>S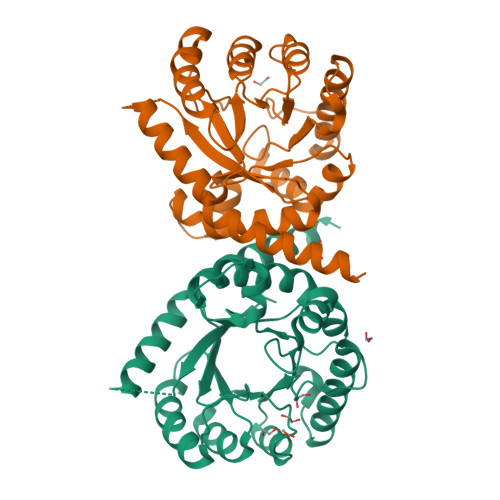NAMTKTKIMGILNVTPDSFSDGGKFNNVETAINRVKAMIDEGADIIDVGGVSTRPGHEMVTLEEELNRVLPVVEAIVGFDVKISVDTFRSEVAEACLKLGVDMINDQWAGLYDHRMFQIVAKYDAEIILMHNGNGNRDEPVVEEMLTSLLAQAHQAKIAGIPSNKIWLDPGIGFAKTRNEEAEVMARLDELVATEYPVLLATSRKRFTKEMMGYDTTPVERDEVTAATTAYGIMKGVRAVRVHNVELNAKLAKGIDFLKENENARHNLS[2x]>MQTSHSLPSAQLPLFQEAFWASNGAPLLDDVIDSPSSASIEEPAAFSELSLSGLPGHCLTLLAPILRELSEEQDARWLTLIAPPASLTHEWLRRAGLNRERILLLQAKDNAAALALSCEALRLGRSHTVVS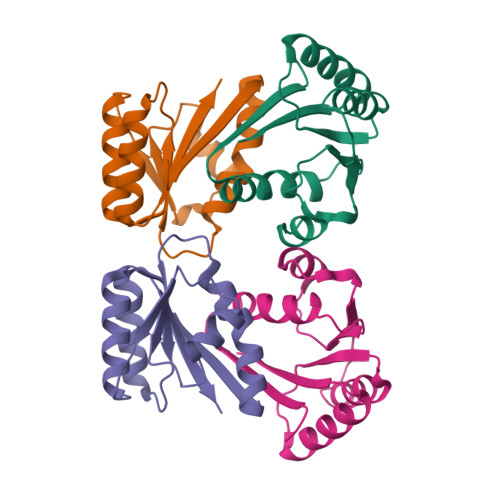WLEPLSRAARKQLSRAAQLGQAQSLNIRLG[4x]TRANDOLAPRILAT | C22 H30 N2 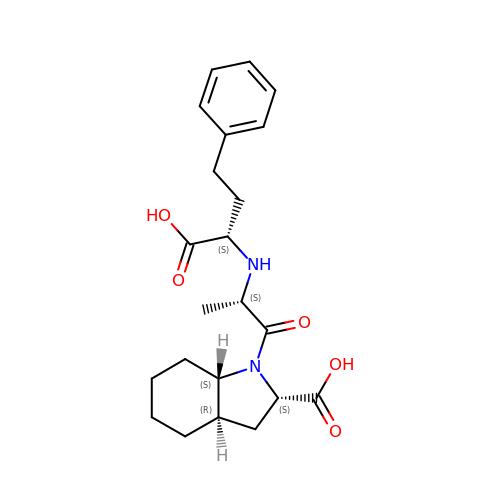O5 | AHYHTSYNOHNUSH-HXFGRODQSA-N>MAGSRQRGLRARVRPLFCALLLSLGRFVRGDGVGGDPAVALPHRRFEYKYSFKGPHLVQSDGTVPFWAHAGNAIPSSDQIRVAPSLKSQRGSVWTKTKAAFENWEVEVTFRVTGRGRIGADGLAIWYAENQGLEGPVFGSADLWNGVGIFFDSFDNDGKKNNPAIVIIGNNGQIHYDHQNDGASQALASCQRDFRNKPYPVRAKITYYQNTLTVMINNGFTPDKNDYEFCAKVENMIIPAQGHFGISAATGGLADDHDVLSFLTFQLTEPGKEPPTPDKEISEKEKEKYQEEFEHFQQELDKKKEEFQKGHPDLQGQPAEEIFESVGDRELRQVFEGQNRIHLEIKQLNRQLDMILDEQRRYVSSLTEEISKRGAGMPGQHGQITQQELDTVVKTQHEILRQVNEMKNSMSETVRLVSGMQHPGSAGGVYETTQHFIDIKEHLHIVKRDIDNLVQRNMPSNEKPKCPELPPFPSCLSTVHFIIFVVVQTVLFIGYIMYRSQQEAAAKKFFGVAMPGAEDDVV[4x];>[4x]GSHMEEPAASFSQPGSMGLDKNTVHDQEHIMEHLEGVINKPEAEMSPQELQLHYFKMHDYDGNNLLDGLELSTAITHVHKEEGSEQAPLMSEDELINIIDGVLRDDDKNNDGYIDYAEFAKSLQ

ERGIC-53 transports certain subsets of newly synthesized secretory proteins and membrane proteins from the endoplasmic reticulum to the Golgi apparatus. MCFD2 is a small protein composed of an EF-hand domain with two Ca2+ binding sites, and functions as a binding partner of ERGIC-53 in a Ca2+-dependent manner. From the amino acid sequence, ERGIC-53 is predicted to be a single-pass transmembrane protein that consists of a luminal carbohydrate recognition domain (CRD), a long stalk domain, a transmembrane (TM) helix and a short cytoplasmic tail (CT). Here we present cryo-EM structures of full-length ERGIC-53 in complex with its functional partner MCFD2. These structures reveal that ERGIC-53 exists as a homotetramer, not a homohexamer as previously suggested, and comprises a four-leaf clover-like head and a long stalk composed of three sets of four-helix coiled-coil followed by a transmembrane domain.

The two different structures of the head region suggest its conformational variability. As observed in forms A and B, component Ihead shows a swing movement of the CRDs, in which the CRD dimer between upper and lower protomers shows a side-to-side rotation as a rigid body dimer. The rotation direction of the dimer is nearly parallel to interface-H (side-to-side rotation).> KDCV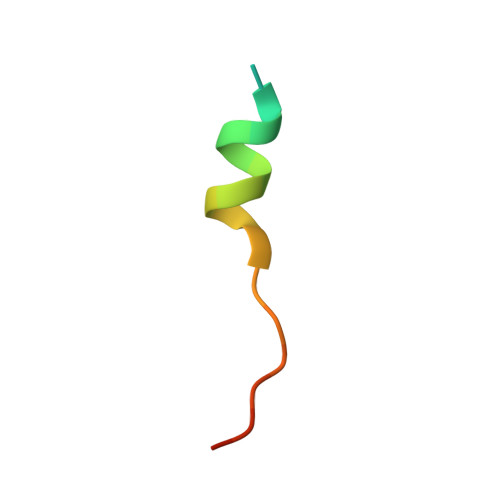FKDWEELGEEIRLKVFVLG>[12x]PRSLANAPIMILNGPNLNLLGQRQPEIYGSDTLADVEALCV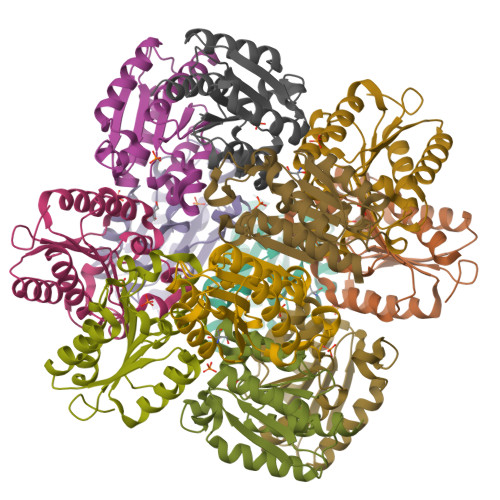KAAAAHGGTVDFRQSNHEGELVDWIHEARLNHCGIVINPAAYSHTSVAILDALNTCDGLPVVEVHISNIHQREPFRHHSYVSQRADGVVAGCGVQGYVFGVERIAALAGAGSARA5-(4-PHENOXYPHENYL)-5-(4-PYRIMIDIN-2-YLPIPERAZIN-1-YL)PYRIMIDINE-2,4,6(2H,3H)-TRIONE 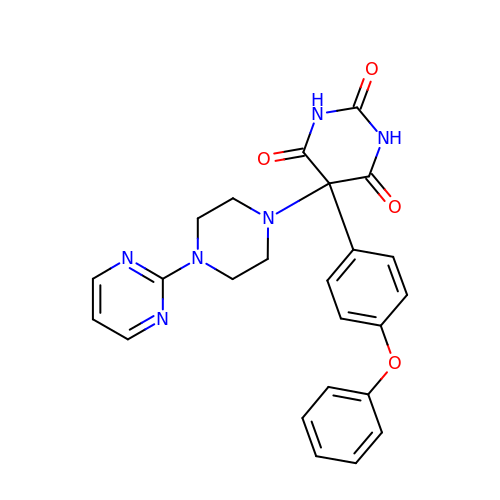| C24 H22 N6 O4 | FMKQJGOROFNCGM-UHFFFAOYSA-N>MTKHKERVMYYGKGDVFAYRTYLKPLTGVRTIPESPFSGRDHILFGVNVKISVGGTKLLTSFTKGDNSLVVATDSMKNFIQKHLASYTGTTIEGFLEYVATSFLKKYSHIEKISLIGEEIPFETTFAVKNGNRAASELVFKKSRNEYATAYLNMVRNEDNTLNITEQQSGLAGLQLIKVSGNSFVGFIRDEYTTLPEDSNRPLFVYLNIKWKYKNTEDSFGTNPENYVAAEQIRDIATSVFHETETLSIQHLIYLIGRRILERFPQLQEVYFESQNHTWDKIVEEIP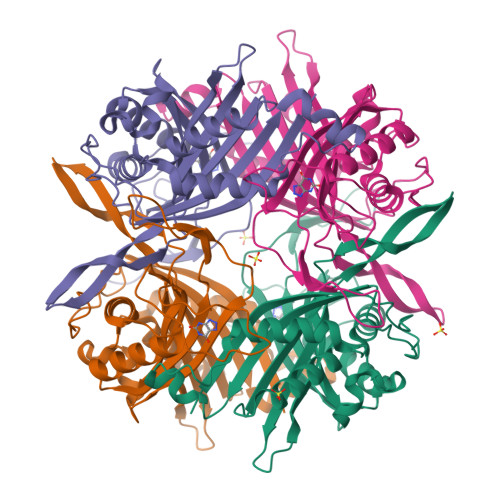ESEGKVYTEPRPPYGFQCFTVTQEDLPHENIL[4x]> MNAIHIGPFSITPAARGLHYGGLPHHQWTLYYGPREMAIKTLPDSYTSSEVRDEFSDIIAEFVIDARHRYAPDVLELVNSDGDAVLARVAVSRLPEALSGCIPDDRFPYWLLTASRPRLGLPVTLNEYTALAVELSAPPLAWITGLLPGEVLTHDAEEWRPPTSWELRHVVGEGSFTGVSGAAAAALLGMSATNFRKYTAGDSAANRQKISFAAWHYLLDRLGVKRASLEH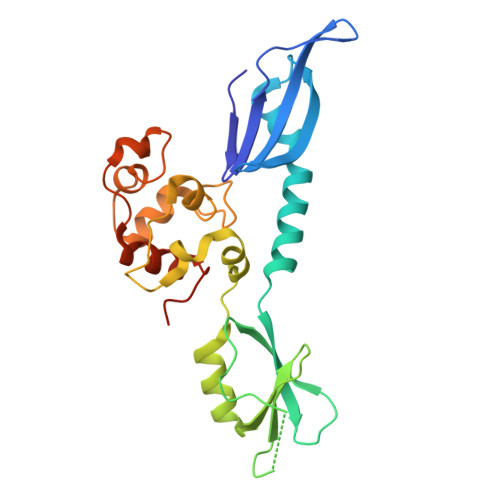HHHHH>[2x]ANLRLSEANSGTYKTFIGRVREELGSETYRLYGIPVLKHSL;>[2x]NRFYLLTLTSNQDESITLAIDVEDMVAVAYQPAGSHESYFFLNAPQIAFHTLFTDTHQNVLNFDNTFKSLENAAGTTRQTIVLGVDPLDFAISNLFNADPKLLPLSFLVIIQMVLEASKFRFIEQSVAYSFKNEKTFLPDLAIVSLEDNWSEISLQIQASTSLQGLFGSVVELYNSNNELIEVDSIYYPIILANVALQLYHCQVST;>[2x]NECLVETRTTRISGRDALCVDVAGALTSDGSRLILYPCGQQVNQKWTFHSDGTVRSLGKCLAT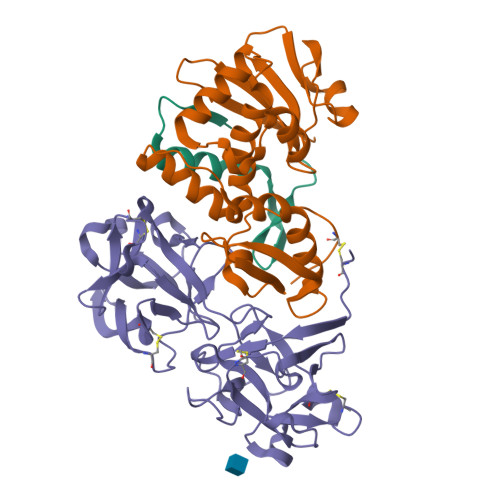NNSKFGNLVVIYDCSKLAAEDISWDVSVGGTIMNPNYEDLALTSNKATRSTNLTMEVNTYSASQGWRVGNYVQPIIGSIVGLDDMCLEATDGNTNMWLEECVPNQREQSWALYSDGTIRVDDNRELCVTASSSTYDNWKVITILNCDGSNNQRWVFLADGSISTPGNQRLAMDVARSDVDLKKIILHRPHGDLNQQWVLFY> 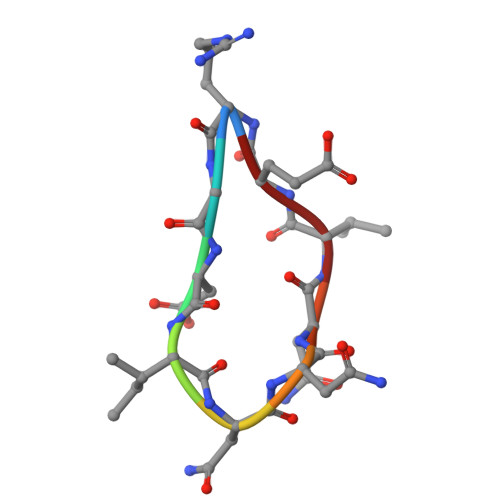RGDINNNVE> SNAAAMSVIDSILDKADEQEIKKLNVIVDKIDALEDSMKNLSYEELKDMTAIFKNRLKKGETLDDILPEAFAVVREVSKRKLGMRQYRVQLIGGIVIHQGKIAEMKTGEGKTLVEVAPVYLNALTGKGVHVITVNDYLAERDKELMSPVYESLGMTVGVIISNQDPNIRKQQYKCDITYGTNSEFGFDYLRDNMVPDLSHKVQRELNFAIVDEVDSILIDEARTPLIIAGDGDEDLKLYELANSFVKTVKEEDFELDRKDKTIALTASGISKAESFFGITNLTDIKNIELYHHINQALRGHKLMEKDVDYVISNGEVMIVDEFTGRVMDGRRYTDGLHQAIEAKEGVEIKNESKTMATVTYQNFFRLYEKLSGMTGTAKTEEGEFESIYKLNVVQIPTNRPVIRADLHDKVFKTEEEKYSAVVEEIIRIHKTRQPILVGTVSVEKSEKLSKMLKKQGIKHQVLNAKQHDKEAEIISKAGKLDAITIATNMAGRGTDISLGAGDK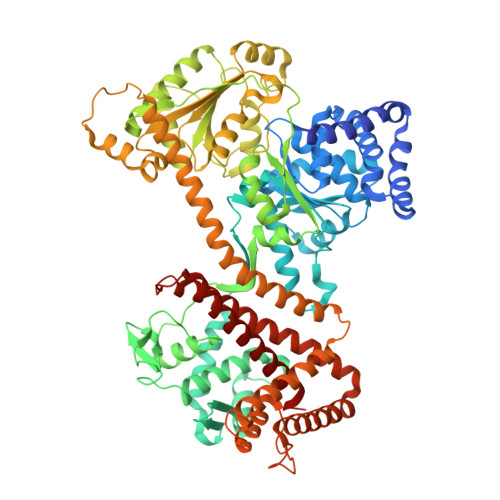EEEQEVKDLGGLYVIGTERHESRRIDNQLRGRSGRQGDPGTSRFFVSLEDDVIKLYGGKTIEKLMKRTSSNENTAIESKALTRAIERAQKGVEGKNFEIRKNVLKYDDTINEQRKVIYNERNKVLNDEDIQEDIQKMVKDIIQEAGETYLIGRKRDYYGYFKHLYSTFMPADTLLIPGVDKKSVQEIIDSTYEISKRVYDLKKMMLGIDKVAELEKTVLLKVVDQYWIDHIDAMEQLKQYIGLKSYAQKDPFKEYALEGYDMFEALNKNIREATVQYLYKFN> MEELDGEPTVTLIPGVNSKKNQMYFDWGPGEMLVCETSFNKKEKSEMVPSCPFIYIIRKDVDVYSQILRKLFNESHGIFLGLQRIDEELTGKSRKSQLVRVSKNYRSVIRACMEEMHQVAIAAKDPANGRQFSSQVSILSAMELIWNLCEILFIEVAPAGPLLLHLLDWVRLHVCEVDSLSADVLGSENPSKHDSFWNLVTILVLQGRLDEARQMLSKEADASPASAGICRIMGDLMRTMPILSPGNTQTLTELELKWQHWHEECERYLQDSTFATSPHLESLLKIMLGDEAALLEQKELLSNWYHFLVTRLLYSNPTVKPIDLHYYAQSSLDLFLGGESSPEPLDNILLAAFEFDIHQVIKECSIALSNWWFVAHLTDLLDHCKLLQSHNLYFGSNMREFLLLEYASGLFAHPSLWQLGVDYFDYCPELGRVSLELHIERIPLNTEQKALKVLRICEQRQMTEQVRSICKILAMKAVRNNRLGSALSWSIRAKDAAFATLVSDRFLRDYCERGCFSDLDLIDNLGPAMMLSDRLTFLGKYREFHRMYGEK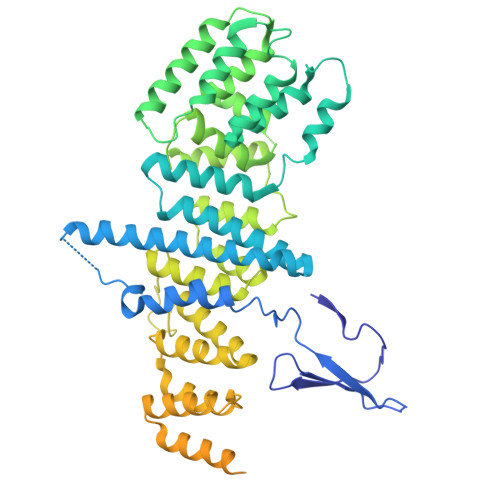RFADAASLLLSLMTSRIAPRSFWMTLLTDALPLLEQKQVIFSAEQTYELMRCLEDLTSRRPVHGESDTEQLQDDDIETTKVEMLRLSLARNLARAIIREGSLEGS>[6x]MKKEKAIVVFSGGQDSTTCLLWALKEFEEVETVTFHYNQRHSQEVEVAKSIAEKLGVKNHLLDMSLLNQLAPNALTRNDIEIEVKDGELPSTFVPGRNLVFLSF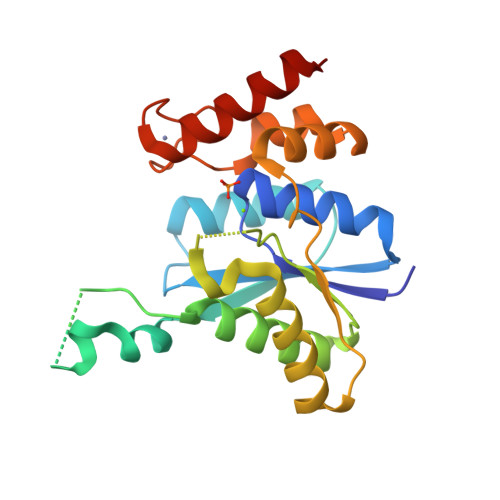ASILAYQIGARHIITGVCETDFSGYPDCRDEFVKSCNVTVNLAMEKPFVIHTPLMWLNKAETWKLADELGALDFVKNNTLTCYNGIIADGCGECPACHLRSKGYEEYMVMKGERA>MENFPTEYFLNTTVRLLEYIRYRDSNYTREERIENLHYAYNKAAHHFAQPRQQQLLKVDPKRLQASLQTIVGMVVYSWAKVSKECMADLSIHYTYTLVLDDSKDDPYPTMVNYFDDLQAGREQAHPWWALVNEHFPNVLRHFGPFCSLNLIRSTLDFFEGCWIEQYNFGGFPGSHDYPQFLRRMNGLGHCVGASLWPKEQFNERSLFLEITSAIAQMENWMVWVNDLMSFYKEFDDERDQISLVKNYVVSDEISLHEALEKLTQDTLHSSKQ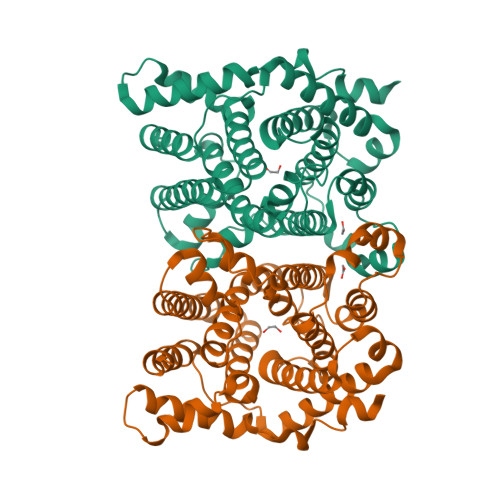MVAVFSDKDPQVMDTIECFMHGYVTWHLCDRRFRLSEIYEKVKEEKTEDAQKFCKFYEQAANVGAVSPSEWAYPPVAQLANVRSKDVKEVQKPFLSSIELVE[2x]3-BENZYL-3-METHYL-5-(1-METHYLPYRAZOL-4-YL)INDOLIN-2-ONE 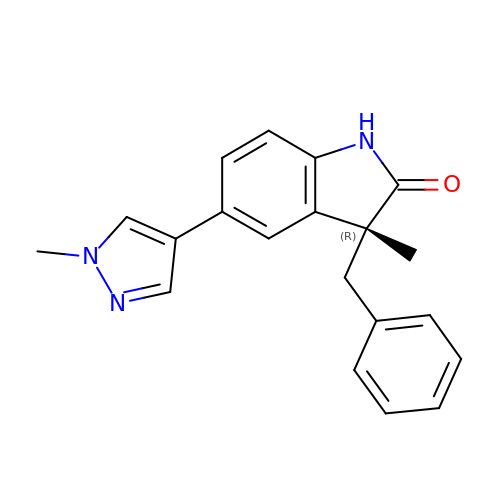| C20 H19 N3 O | PXFSEAGTJRSUCG-HXUWFJFHSA-N CLC-2 is a voltage-gated chloride channel that contributes to electrical excitability and ion homeostasis in many different tissues. Among the nine mammalian CLC homologs, CLC-2 is uniquely activated by hyperpolarization, rather than depolarization, of the plasma membrane. The TM region of CLC-2 displays a typical CLC family symmetric homodimeric structure, with each subunit containing an independent Cl− pathway. All eukaryotic CLCs contain a pair of ‘cystathionine β-synthase’ (CBS) domains in their intracellular C-terminal domain (CTD).

Selected two-dimensional class averages showed a clear TM domain embedded in a detergent micelle and features indicating an intracellular domain. Further refinement revealed a well-resolved TM domain density at 2.46 Å, ‘CLC2-TM’ (Figure 2—figure supplements 1–3). In the cryoEM map, clear density for the Egate residue (E205 in CLC-2) reveals it occupying the ‘down’ position, at the Scen Cl−-binding site. Our cryoEM map also reveals a density feature at the Sext site, consistent with a bound Cl− ion. First, Egate physically occupies the Scen Cl−-binding site, thus blocking the permeation pathway. The pinch point of ~0.7 Å near the Egate residue is too narrow for a Cl− ion and thus indicates a closed conformational state. CLC-2 is the first CLC channel homolog to be seen in a closed conformational state. Another new feature of the determined CLC-2 structure is a hairpin density blocking the main Cl− pathway on the intracellular side. We tested several candidate fragments from the CLC-2 N-terminal region and found that the hairpin density fits perfectly with residues corresponding to 14–28. The hairpin structure appears to directly block the pore. CLC-2 also displays a bifurcated pore, with a secondary pathway to the intracellular side, distinct from the primary pathway common to CLC family members.

>[2x]MAAAAAEEGMEPRALQYEQTLMYGRYTQDLGAFAKEEAARIRLGGPEPWKGPPSSRAAPELLEYGRSRCARCRVCSVRCHKFLVSRVGEDWIFLVLLGLLMALVSWVMDYAIAACLQAQQWMSRGLNTSILLQYLAWVTYPVVLITFSAGFTQILAPQAVGSGIPEMKTILRGVVLKEYLTLKTFIAKVIGLTCALGSGMPLGKEGPFVHIASMCAALLSKFLSLFGGIYENESRNTEMLAAACAVGVGCCFAAPIGGVLFSIEVTSTFFAVRNYWRGFFAATFSAFIFRVLAVWNRDEETITALFKTRFRLDFPFDLQELPAFAVIGIASGFGGALFVYLNRKIVQVMRKQKTINRFLMRKRLLFPALVTLLISTLTFPPGFGQFMAGQLSQKETLVTLFDNRTWVRQGLVEELEPPSTSQAWNPPRANVFLTLVIFILMKFWMSALATTIPVPCGAFMPVFVIGAAFGRLVGESMAAWFPDGIHTDSSTYRIVPGGYAVVGAAALAGAVTHTVSTAVIVFELTGQIAHILPVMIAVILANAVAQSLQPSLYDSIIRIKKLPYLPELGWGRHQQYRVRVEDIMVRDVPHVALSCTFRDLRLALHRTKGRMLALVESPESMILLGSIERSQVVALLGAQLSPARRRQHMQERRATQTSPLSDQEGPPSPEASVCFQVNTEDSAFPAARGETHKPLKPALKRGPSVTRNLGESPTGSAESAGIALRSLFCGSPPPEAASEKLESCEKRKLKRVRISLASDADLEGEMSPEEILEWEEQQLDEPVNFSDCKIDPAPFQLVERTSLHKLRKAIEGSVTAQGVKVRPPLASFRDSATSSSDTETTEVHALWGPHSRHGLPREGSPSDSDDKCQ>ACUCGUUUGAGCGAGUAUAAACAGCUGGUUAAGCUCAAAGCGGAGA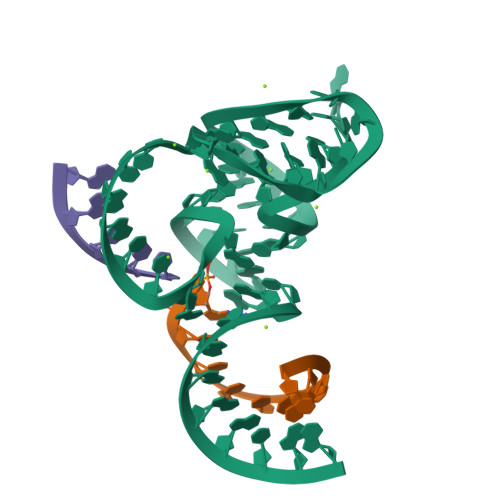GCAGA[2x];>UCUGCUCUCX[2x];>[2x]UCCAG> GPLGSIKELAVDEELAAADGLIPRQKSKLCKHGDRGMCEYCSPLPPWDKEYHEKNKIKHISFHSYLKKLNENANKKENGSSYISPLSEPDFRINKRCHNGHEPWPRGICSKCQPSAITLQQQEFRMVDHVEFQKSEIINEFIQAWRYTGMQRFGYMYGSYSKYDNTPLGIKAVVEAIYEPPQHDEQDGLTMDVEQVKNEML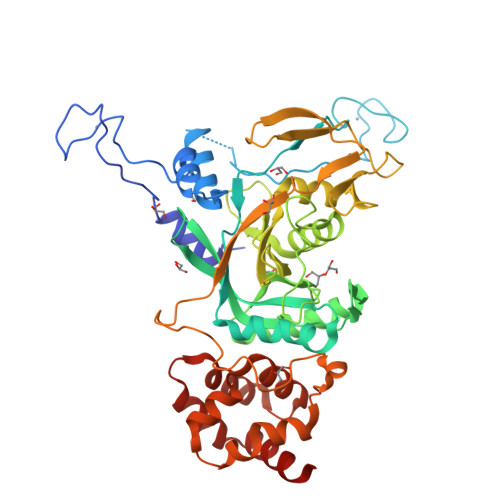QIDRQAQEMGLSRIGLIFTDLSDAGAGDGSVFCKRHKDSFFLSSLEVIMAARHQTRHPNVSKYSEQGFFSSKFVTCVISGNLEGEIDISSYQVSTEAEALVTADMISGSTFPSMAYINDTTDERYVPEIFYMKSNEYGITVKENAKPAFPVDYLLVTLTHGFPNTDTETNSKFVSSTGFPWSNRQAMGQSQDYQELKKYLFNVASSGDFNLLHEKISNFHLLLYINSLQILSPDEWKLLIESAVKNEWEESLLKLVSSAGWQTLVMILQESG(4S)-4-AMINO-5-HYDROXYPENTANOIC ACID | C5 H11 N O3 | 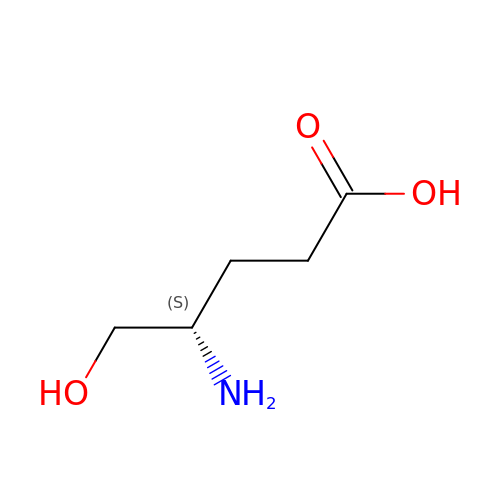JPYGFLFUDLRNKX-BYPYZUCNSA-N> FAGGIVSQRCLSCICKMESGCRNV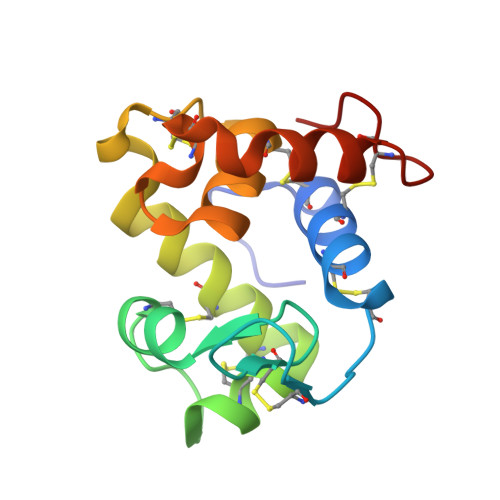GCKMDMGSLSCGYFQIKEAYWIDCGRPGSSWKSCAASSYCASLCVQNYMKRYAKWAGCPLRCEGFAREHNGGPRGCKKGSTIGYWNRLQKISGCHGVQ>[3x]GPGGSMKRLRPSDKFFELLGYKPHHVQLAIHRSTAKRRVACLGRQSGKSEAASVEAVFELFARPGSQGWIIAP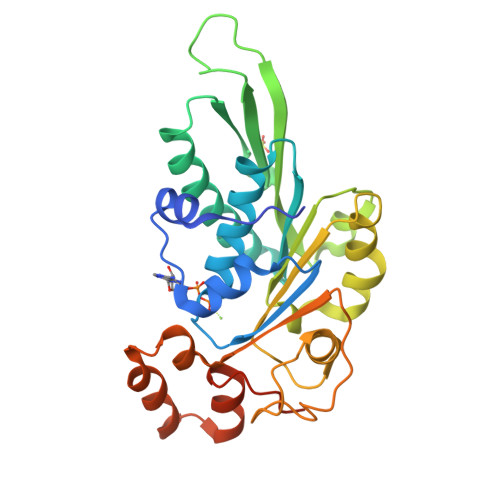TYDQAEIIFGRVVEKVERLAEVFPATEVQLQRRRLRLLVHHYDRPVNAPGAKRVATSEFRGKSADRPDNLRGATLDFVILDEAAMIPFSVWSEAIEPTLSVRDGWALIISTPKGLNWFYEFFLMGWRGGLKEGIPNSGINQTHPDFESFHAASWDVWPERREWYMERRLYIPDLEFRQEYGAEFVSHSGLEHHHHHHHHHH>MTHHYPTDDIKIKEVKELLPPIAHLYELPISKEASGLVHRTRQEISDLVHGRDKRLLVIIG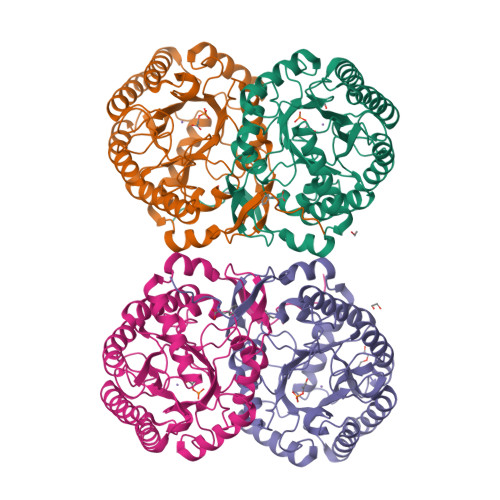PCSIHDPKAALEYAERLLKLRKQYENELLIVMRVYFAKPRTTVGWKGLINDPHLDGTFDINFGLRQARSLLLSLNNMGMPASTEFLDMITPQYYADLISWGAIGARTTESQVHRELASGLSCPVGFKNGTDGNLKIAIDAIGAASHSHHFLSVTKAGHSAIVHTGGNPDCHVILRGGKEPNYDAEHVSEAAEQLRAAGVTDKLMIDCSHANSRKDYTRQMEVAQDIAAQLEQDGGNIMGVMVESHLVEGRQDKPEVYGKSITDACIGWGATEELLALLAGANKKRMARAS[4x]> MGHHHHHHENLYFQGHMTLAVKVPLKEGEIVRRRLIELGALDNTYKIKREGNFLLIPVKFPVKGFEVVEAELEQVSRRPNSYREIVNVPQELRRFLPTSFDIIGNIAIIEIPEELKGYAKEIGRAIVEVHKNVKAVYMKGSKIEGEYRTRELIHIAGENITETIHRENGIRLKLDVAKVYFSPRLATERMRVFKMAQEGEVVFDMFAGVGPFSILLAKKAELVFACDINPWAIKYLEENIKLNKVNNVVPILGDSREIEVKADRIIMNLPKYAHEFLEHAISCINDGGVIHYYGFGPEGDPYGWHLERIRELANKFGVK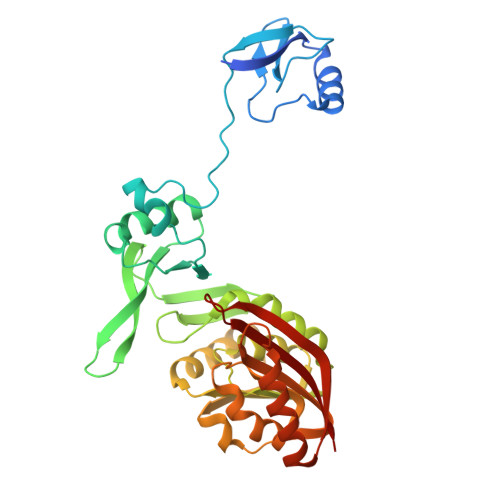VEVLGKRVIRNYAPRQYNIAIDFRVSF> PFIECHIATGLSVARKQQLIRDVIDVTNKSIGSDPKIINVL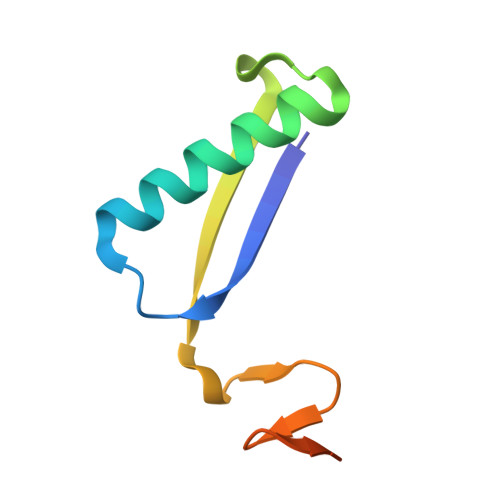LVEHAEANMSISGRIHGEAASTERTPAVS{1-[2-(1-FORMYL-PROPYL)-3-METHANESULFONYLAMINO-PYRROLIDINE-1-CARBONYL]-2-METHYL-PROPYL}-CARBAMIC ACID TERT-BUTYL ESTER | C19 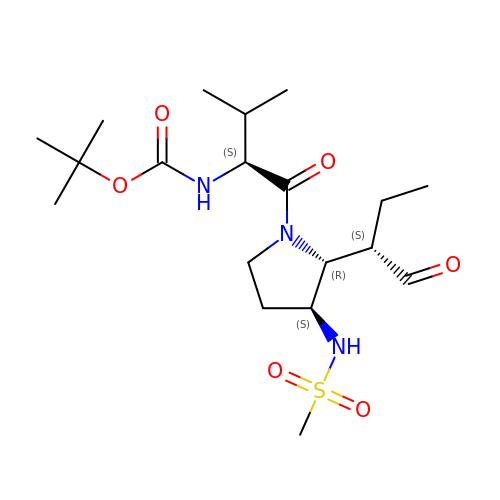H35 N3 O6 S | NOWIRVOXJOWTSQ-FXUDXRNXSA-N>ADNRRPIWNLAHMVNAVAQIPDFLDLGANALEADVTFKGSVPTYTYHGTPCDFGRDCIRWEYFNVFLKTLREYTTPGNAKYRDGFILFVLDLKTGSLSNDQVRPAGENVAKELLQNYWNNGNNGGRAYVVLSLPDIGHYEFVRGFKEVLKKEGHEDLLEKVGYDFSGPYLPSL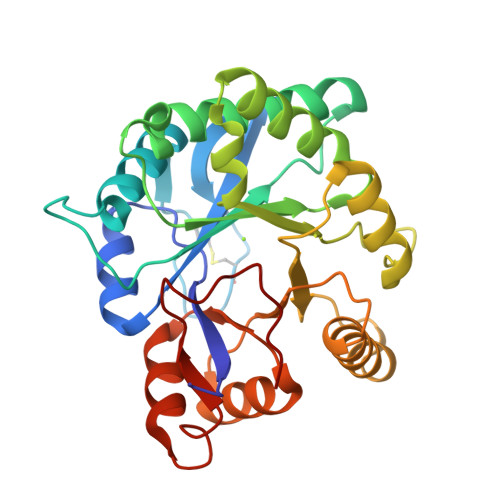PTLDATHEAYKKAGVDGHIWLSDGLTNFSPLGDMARLKEAIKSRDSANGFINKIYYWSVDKVSTTKAALDVGVDGIMTNYPNVLIGVLKESGYNDKYRLATYDDNPWETFKN[4x]>[4x]ETLVRPKPELLKLLKSVGAQKDTYTMKEVLFYLGQY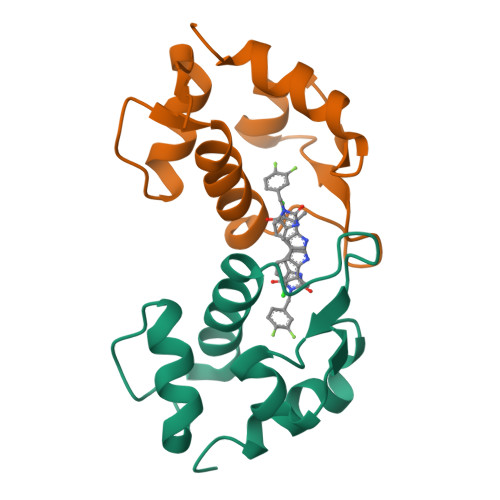IMTKRLYDEKQQHIVYCSNDLLGDLFGVPSFSVKEHRKIYTMIYRNLVV>[7x]GSMAKVQVNNVVVLDNPSPFYNPFQFEITFECIEDLSEDLEWKIIYVGSAESEEYDQVLDSVLVGPVPAGRHMFVFQADAPNPGLIPDADAVGVTVVLITCTYRGQEFIRVGYYVNNEYTETELRENPPVKPDFSKLQRNILASNPRVTRFHINWED

By binding histone H3–H4 dimers, the histone chaperone ASF1 facilitates nucleosome assembly and turnover and modulates histone post-translational modifications. ASF1 consists of an N-terminal 155-residue immunoglobulin-like domain (ASF1-NT) followed by a presumably unstructured C-terminal tail. As expected from prior structures of human and yeast ASF119,20,59, ASF1a-NT adopted an immunoglobulin (Ig) domain-like fold, composed of a β sandwich topped by α helices. Specifically, phosphorylation of the C-terminal tail of histone-free ASF1 by tousled-like kinases (TLKs) increases its association with the H3–H4 dimer and downstream chaperones, which has been suggested to promote the provision of histones for chromatin assembly.

In order to determine how TLK2 engages ASF1a, we determined the crystal structure of the human ASF1a NT domain in the presence and absence of the N-terminal TLK2 peptide. Apo-ASF1a-NT crystallized in space group C2 with seven molecules in the asymmetric unit, while the complex with the TLK2 peptide crystalized in the P21 space group with eight complexes in the asymmetric unit. The structure of apo-ASF1 NT domain was resolved to 2.1 Å and in complex with the TLK2 peptide to 2.71 Å. The ASF1a structure exhibited little variation between the chains in each structure, with an average root mean square deviation (RMSD) of 0.65 Å between 153–155 residues for the seven chains in the apo-ASF1a structure and RMSD of 0.39 Å over 151–154 residues among the eight ASF1a chains in the ASF1a·TLK2 peptide complex structure. Notably, aside from re-orientation of side chains interacting with the TLK2 peptide, the ASF1a Ig-like domain did not display any significant structural changes between the apo and complex form, with an average RMSD of 0.59 Å over 151–154 residues between chain A of apo-ASF1a structure and the eight ASF1a chains of the ASF1a·TLK2 structure.>[2x]MKLQVLPLSQEAFSAYGDVIETQQRDFFHINNGLVERYHDLALVEILEQDRTLISINRAQPANLPLTIHELERHPLGTQA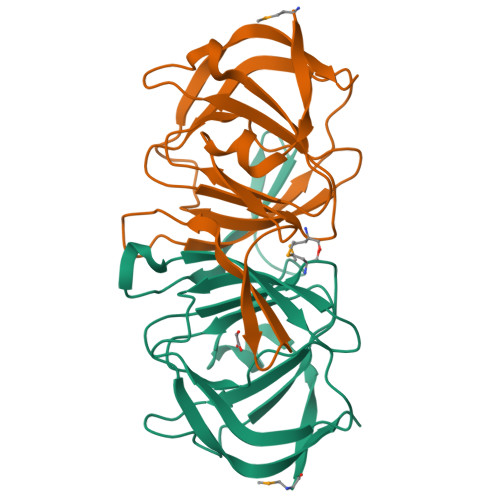FIPMKGEVFVVVVALGDDKPDLSTLRAFITNGEQGVNYHRNVWHHPLFAWQRVTDFLTIDRGGSDNCDVESIPEQELCFAGSHHHHHHHH>[2x]GSHMVRNVDVKSRIMDQYADWKGVRYRLGGSTKKGIDSSGFVQRTFR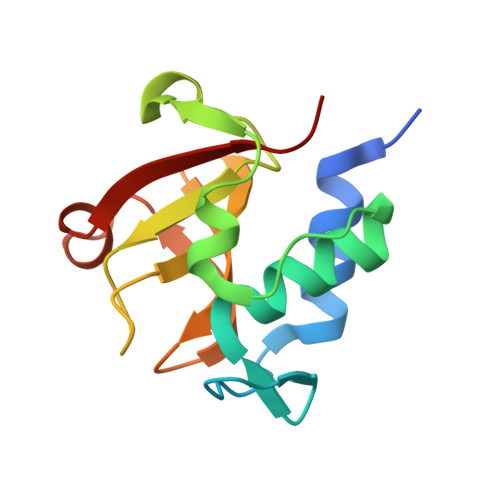EQFGLELPRSTYEQQEMGKSVSRSNLRTGDLVLFRAGSTGRHVGIYIGNNQFVHASTSSGVIISSMNEPYWKKRYNEARRVLSRS> MVYPVRNKDDLDQQLILAEDKLVVIDFYADWCGPCKIIAPKLDELAHEYSDRVVVLKVNVDENEDITVEYNVNSMPTFVFIKGGNVLELFVGCN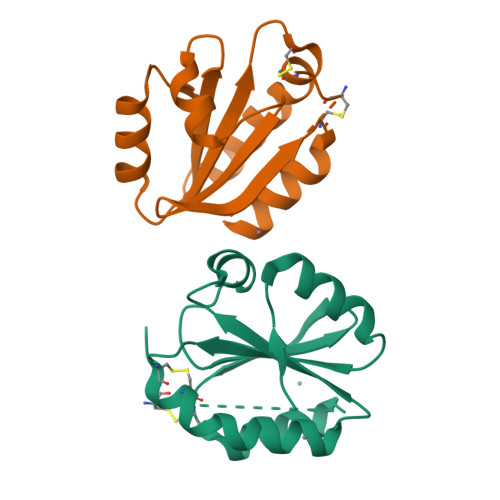SDKLAKLMEKHAGVYTDEAADVKAVHIDGECIVDLTAESSESDNDNNNVNEVSAHDENAVLEH(3E,5E)-6-(4-nitrophenyl)-2-oxohexa-3,5-dienoic acid | C12 H9 N O5 | 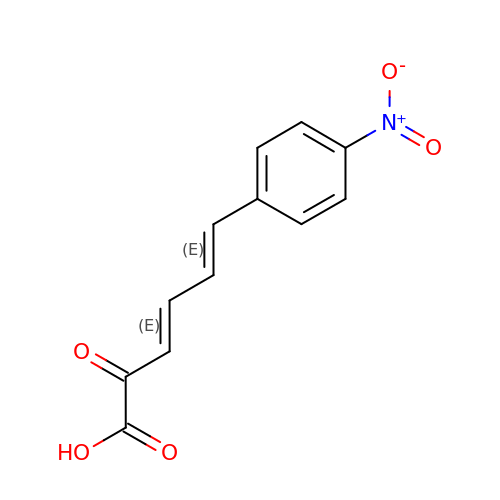YFKMPGYOVOFESP-ZPUQHVIOSA-N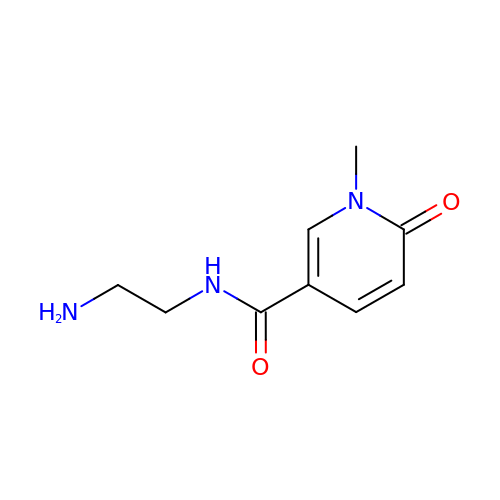~{N}-(2-azanylethyl)-1-methyl-6-oxidanylidene-pyridine-3-carboxamide | C9 H13 N3 O2 | MBASUXNNJWJUFS-UHFFFAOYSA-N Human NAD-dependent isocitrate dehydrogenase or IDH3 (HsIDH3) catalyzes the decarboxylation of isocitrate into α-ketoglutarate in the tricarboxylic acid cycle. It consists of three types of subunits (α, β, and γ) and exists and functions as the (αβαγ)2 heterooctamer. HsIDH3 is regulated allosterically and/or competitively by numerous metabolites including CIT, ADP, ATP, and NADH. In this work, we report the crystal structures of the αβ and αγ heterodimers and the (αβαγ)2 heterooctamer containing an α-Q139A mutation in the clasp domain, which renders all the heterodimers and the heterooctamer constitutively active in the absence of activators.

Crystals of αMICT+Ca+NADβNAD belong to space group C2221 and there are two αMβ heterodimers in an asymmetry unit, which form an (αMβ)2 heterotetramer through a noncrystallographic 2-fold axis. In this structure, there are an ICT, NAD, and Ca2+ bound at the active site of the α subunit, which are clearly defined in the electron density map; in addition, there is an NAD bound at the pseudo-allosteric site of the β subunit, and the ADP-ribose moiety of NAD is well defined in the electron density map albeit the nicotinamide moiety is poor defined. In the αMICT+Ca+NADβNAD structure, the active site is bound with the substrate ICT, the cofactor NAD, and a Ca2+ ion. This is the first pseudo-Michaelis complex reported for HsIDH3 and other NAD-IDHs. In contrast, compared to that in the αMβ structure, the α large domain in the αMICT+Ca+NADβNAD structure exhibits a 6° rotation toward the α-β interface owing to the binding of ICT and NAD, resulting in a “closed” conformation of the active site (see Discussion later). The binding of NAD to the active site induces the α large domain and in particular, the β3A-α3A and β12A-α8A loops to rotate toward the α-β interface, resulting in a closed conformation of the active site. In contrast, in the αMICT+Ca+NADβNAD structure, the N-terminal regions of the α7 helices adopt the active helical conformations and the sidechain of Tyr126A also adopts the active conformation, which lead the sidechains of Asp230A, Asp234A, and Asp217B in proper orientations to form coordination bonds with the Ca2+ ion. In addition, the sidechain of Asp230A is in close proximity to the hydroxyl group of Tyr126A (2.8 Å) and the ε-ammonium group of Lys184B (2.9 Å). Thus, the Lys184B-Asp230A-Tyr126A triad appears to be in favorable geometries for proton transfer. Specifically, the α-carboxyl group interacts with Arg88A, Arg98A, and Arg119A; the β-carboxyl group interacts with Arg88A and Arg119A; the γ-carboxyl group interacts with Thr74A, Ser82A, Asn84A; and the α-hydroxyl group forms hydrogen bonds with Lys184B, Asp217B, and Asp230A, and a coordination bond with the Ca2+ ion.

>[2x]TGGVQTVTLIPGDGIGPEISAAVMKIFDAAKAPIQWEERNVTAIQGPGGKWMIPSEAKESMDKNKMGLKGPLKTPIAAGHPSMNLLLRKTFDLYANVRPCVSIEGYKTPYTDVNIVTIRENTEGEYSGIEHVIVDGVVASIKLITEGASKRIAEFAFEYARNNHRSNVTAVHKANIMRMSDGLFLQKCREVAESCKDIKFNEMYLDTVCLNMVQDPSQFDVLVMPNLYGDILSDLCAGLIGGLGVTPSGNIGANGVAIFESVHGTAPDIAGKDMANPTALLLSAVMMLRHMGLFDHAARIEAACFATIKDGKSLTKDLGGNAKCSDFTEEICRRVKDLD;>[2x]ASRSQAEDVRVEGSFPVTMLPGDGVGPELMHAVKEVFKAAAVPVEFQEHHLSEVQNMASEEKLEQVLSSMKENKVAIIGKIHTPMEYKGELASYDMRLRRKLDLFANVVHVKSLPGYMTRHNNLDLVIIREQTEGEYSSLEHESARGVIECLKIVTRAKSQRIAKFAFDYATKKGRGKVTAVHKANIMKLGDGLFLQCCEEVAELYPKIKFETMIIDNCCMQLVQNPYQFDVLVMPNLYGNIIDNLAAGLVGGAGVVPGESYSAEYAVFETGARHPFAQAVGRNIANPTAMLLSASNMLRHLNLEYHSSMIADAVKKVIKVGKVRTSDMGGYATCHDFTEEICRRVKDLDEN> SNAMTNSSEKQWERIQQLEKEHVEVYRELLITLDRLYLIRKHNHAVILSHTQQRLLEIRHQLQINLEKTALLIRLLEKPDNTNVLFTKLQNLLEESNSLDYELLQSLGAQSSLHKQLIESRAERDELMSKLIELSSKFPKPTIPPDDSDTAGKQVEVEKENETIQELMIALQIHSGYTNISYTI;> SNAMSLILDDIILSLTNANERTPPQALKTTLSLLYEKSKQYGLSSPQLQALVRLLCETSIIDTVTKVYIVENCFLPDGYLTKELLLEIINHLGTPTVFSRYRI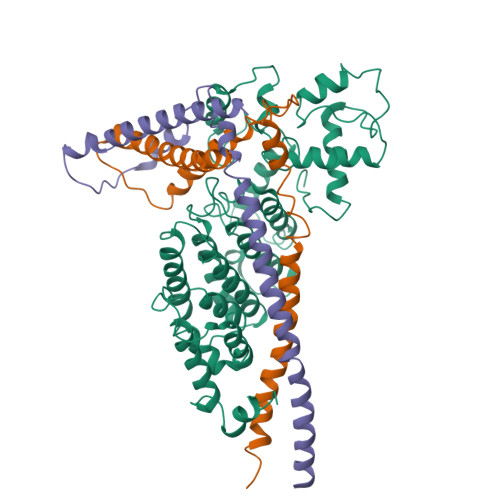QTPPVLQSALCKWLVHVYFLFPVHSEREHNISSSIWLHLWQFSFLQKWITPLVIWQATTPVDVKPWKLSIIKRCAMHPGYRDAPGSATLILQRFQCLVGASSQITESIITINCNRKTLKSHRNLKLDAHFLSILKRILSRAHPANFPADTVQNTIDMYLSEIHQLGADSIYPLRLQSLPEYVPSDSTVSLWDVTSLEQLAQNWPQLHIPNDVDYMMKPSLNSNVLLPRKVMSRDSLKHLYSSIILIKNSRDESSSPYEWCIWQLKRCFAHQIETPQEVIPIIISVSSMDNKLSSRIIQTFCNLKYLKLDELTLKKVCGGILPLWKPELISGTREFFVKFMASIFMWSTRDGHDNNCTFSETCFYVLQMITNWVLDDKLIALGLTLLHDMQSLLTLDKIFNNATSNRFSTMAFISSLDILTQLSKQTKSDYAIQYLIVGPDIMNKVFSSDDPLLLSAACRYLVATKNKLMQYPSTNKFVRMQNQYIMDLTNYLYRNKVLSSKSLFGVSPDFFKQILENLYIPTADFKNAKFFTITGIPALSYICIIILRRLETAENTKIKFTSGIINEETFNNFFRVHHDEIGQHGWIKGVNNIHDLRVKILMHLSNTANPYRDIAAFLFTYLKSLSKYSVQNS;> SNAMDVEKDVLDVYIKNLENQIGNKRYFLKQAQGAIDEITKRSLDTEGKPVNSEVFTELLRKPMFFSERADPIGFSLTSNFLSLRAQSSSEWLSLMNDQSVDQKAMLLLQNNINSDLKELLRKLQHQMTIMDSKKQDHAHIRTRKARNKELWDSLADFLKGYLVPNLDDNDESIDSLTNEVMLLMKRLIEHDLNLTLNDFSSKTIPIYRLLLRANIITVIEGSTNPGTKYIKLIDFNETSLT> AEQKTLHIYNWTDYIAPDTVANFEKETGIKVVYDVFDSNEVLEGKLMAGSTGFDLVVPSASFLERQLTAGVFQPLDKSKLPEWKNLDPELLKLVAKHDPDNKFAMPYMWATTGIGYNVDKVKAVLGENAPVDSWDLILKPENLEKLKSCGVSFLDDPEEVFATVLNYLGKDPNSTKADDYTGPATDLLLKLRPNIRYFHSSQYINDLANGDICVAIGWAGSVWQASNRAKEAKNGVNVSFSIPKEGAMAWFDVFAMPADAKNKDEAYQFLNYLLRPDVVAHISDHVFYANANKAATPLVSAEVRENPGIYPPADVRAKLFTQKVQDPKIDRVRTRAWTKVKSGKLEHHHHHH

To gain insight into the evolution and designability of ligand binding and specificity, we analyzed the homologous PBPs, PotF and PotD, which are Escherichia coli putrescine (PUT)-binding protein and spermidine (SPD)-binding protein, respectively. They constitute the first elements of two separate multicomponent uptake systems (PotFGHI and PotABCD) to transport the cationic polyamines PUT and SPD across the cellular membrane. Still, the protein-binding modes differ: PotF shows affinity for PUT and SPD, whereas PotD exclusively binds SPD. Prior to this work, we grafted the seven differences in amino acids from PotD binding pocket onto PotF; this resulted in PotF_SPD, which will be referred to as PotF/D throughout this work to keep naming for mutants more concise.

All prior observations combined led to the following three constructs: the basic double salt bridge reintroduction E39D–Y87S as well as E39D–F88A and E39D–Y87S–F88Y. Upon analysis by ITC, an increased SPD affinity was observed for each of the constructed variants. Binding modes of constructs containing Y87S are again similar to the SPD binding of PotFs, revealing beneficial enthalpic and entropic shares. To our surprise, all solved structures adopt a PotF/D-like semiclosed conformation. Also, SPD adopts similar positions to the one in PotF/D in all structures. In E39D–Y87S, no specific differences to PotF/D are observable. In the E39D–Y87S structure, R91 shows an additional alternate conformation that can interact with E69. The respective R254 can partially interact with D39 and N231. This time, R254 adopts an alternative conformation in E39D–Y87S and E39D–F88L, favoring one of the possible interactions in each, respectively.> MPAEIDIDEADVLVLSQELQKTSKLTFEINKSLKKIAATSNQSSQLFTPILARNNVLTTLQRNIESTLNSVASVKDLANEASKYEIILQKGINQVGLKQYTQVVHKLDDMLEDIQSGQANREENSEFHGILTHLEQLIKRSEAQLRVYFISILNSIKPFDPQINITKKMPFPYYEDQQLGALSWILDYFHGNSEGSIIQDILVGERSKLILKCMAFLEPFAKEISTAKNAPYEKGSSGMNSYTEALLGFIANEKSLVDDLYSQYTESKPHVLSQILSPLISAYAKLFGANLKIVRSNLENFGFFSFELVESINDVKKSLRGKELQNYNLLQDCTQEVRQVTQSLFRDAIDRIIKKANSISTIPSNNGVTEATVDTMSRLRKFSEYKNGCLGAMDNITRENWLPSNYKEKEYTLQNEALNWEDHNVLLSCFISDCIDTLAVNLERKAQIALMPNQEPDVANPNSSKNKHKQRIG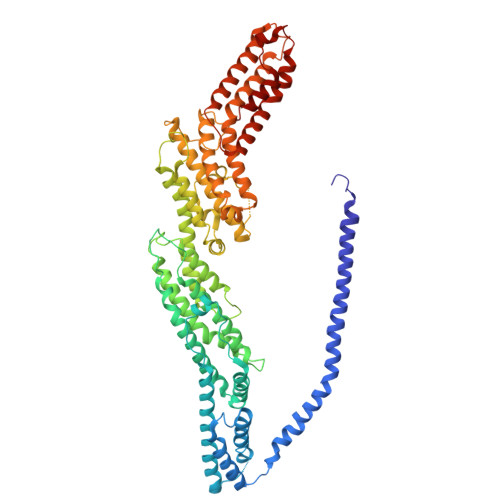FFILMNLTLVEQIVEKSELNLMLAGEGHSRLERLKKRYISYMVSDWRDLTANLMDSVFIDSSGKKSKDKEQIKEKFRKFNEGFEDLVSKTKQYKLSDPSLKVTLKSEIISLVMPMYERFYSRYKDSFKNPRKHIKYTPDELTTVLNQLVR9-METHYL URIC ACID | C6 H6 N4 O3 | 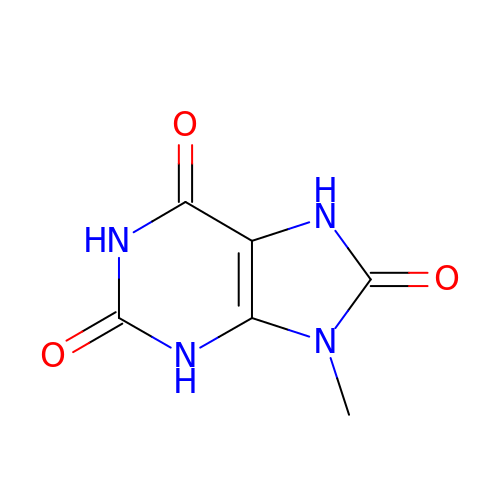XJEJWDFDVPDMAS-UHFFFAOYSA-N(2S)-2,3-dihydroxypropyl 2-acetamido-2-deoxy-alpha-D-glucopyranoside 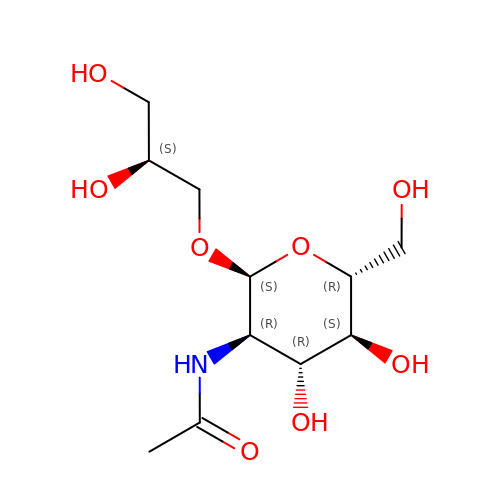| C11 H21 N O8 | BURZSZGRQNCGQJ-KEWAQLPFSA-N>[2x]MSGAPPPSSGFAPRSYGQQPLSHAPRSSMMSVEYDGIPLPPPSIRSCGSQQYVTSYIPTGAAFPPSSVQDMISSMKSYASATDLVRTYSEIPSVEEALSTLDRAAAALNARRYRDALKLYLEGGYAMANVAERQANPKICNLLTSKGFETLNWCARLCDWIEGRIKEKHPRPGVHKVGIPVSNWDEDWVGPFMDEEEARRMWYTPVYCPHPIDFSNLGYRLRCVETGRRPRLMICITMYNEGPQQLKATLKKLANNLAYLKEQMPGDEKSLTGAFAGDDVWQNVLVCIVADGREQVHPKTLDYLEAIGLYDEDLLTINSAGIGAQCHLFEHTLQLSVNGKCLLPIQTVFALKENKASKLDSHHWYFNAFAEQIQPEYTAVMDVGTMLTKSALYHLLFAFERNHQIGGACGQLTVDNPFENLSNWVISAQHFEYKISNILDKSLESCFGFISVLPGAFSAYRYEAIRGAPLDAYFQTLNIELDVLGPFIGNMYLAADRILSFEVVARKNCNWTMHYVKDAVARTDVPHDLVGLISQRKRWLNGAFFATLFSIWNWGRIYSESKHTFVRKMAFLVFYVYHLLYTAFGFFLPANLYLALFFIVFQGFQQNRLEFIDTSEYSQTVLDCAVYIYNFSYLFGLLMLIIIGLGNNPKHMKLTYYFVGAVFGLMMMLSSLVGAGIFFSTPATVHSIVVSILTVGVYFIASALHGEVHHIFMTFTHYTALIPSFVNIFTIYSFCNLQDLSWGTKGLHDDPLLAASLDETEKGDFKDVIAKRRALEELRREEKERVENRKKNFEAFRTNVLLTWAFSNLIFALFVVYFASSSTYMPVLYIFVASLNTCRLLGSIGHWVYIHTEGLRGRVIDKSECGNGTGRYPQNSYVQLEEHYAALAEDQRTYASGRTNASVRTVNDVSSAA

The core of the chitin biosynthetic machinery is an integral membrane enzyme named chitin synthase (CHS) (EC 2.4.1.16). Here we report five cryo-electron microscopy structures of a chitin synthase from the devastating soybean root rot pathogenic oomycete Phytophthora sojae (PsChs1). They represent the apo, GlcNAc-bound, nascent chitin oligomer-bound, UDP-bound (post-synthesis) and chitin synthase inhibitor nikkomycin Z-bound states of the enzyme, providing detailed views into the multiple steps of chitin biosynthesis and its competitive inhibition. The structures reveal the chitin synthesis reaction chamber that has the substrate-binding site, the catalytic centre and the entrance to the polymer-translocating channel that allows the product polymer to be discharged.

To obtain the donor substrate UDP-GlcNAc-bound structure, we mutated the catalytically important residue Glu495 to alanine, which allows the enzyme to trap the substrate in its substrate-binding site. The uridine moiety of UDP-GlcNAc is fixed within the tub of the reaction chamber, which consists of a loop region from Thr237 to Glu241 in the GT domain of the enzyme, through a series of interactions with the residues in this region. The GlcNAc moiety appears to be solvent-exposed and oriented away from the catalytic site. Superposition of UDP-GlcNAc-bound PsChs1 with apo-PsChs1 showed no significant local or global structural differences (root mean square deviation of 0.54 Å for 693 Cα atoms). An N-terminal sequence (residues 23–39), unresolved in the PsChs1 apo structure, appeared as an α-helix in the UDP-GlcNAc complex. This helix extends into the opposite protomer and interacts with the LG subdomain through hydrogen bonds. Structural comparison between the apo and UDP-GlcNAc-bound states revealed that residues Pro38, Leu39 and Pro40 are in different locations, indicating that the N-terminal extension of the SP subdomain in the UDP-GlcNAc-bound state adopts a different conformation. The Mn2+ ion in the UDP-GlcNAc-bound structure only forms charge interaction with the phosphate groups, with a bond distance of more than 3.5 Å, which is much weaker than a coordinate bond. The donor substrate-bound structure shows an additional N-terminal region from residues 23–39. It forms charge interactions with the diphosphate group of either UDP-GlcNAc or UDP in all the substrate-bound, product-bound and UDP-bound structures.>[4x]SRTDRLEVCREYQR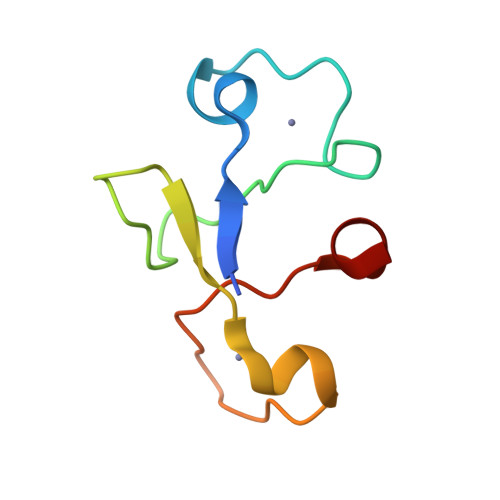GNCNRGENDCRFAHPADSTMIDTNDNTVTVCMDYIKGRCSREKCKYFHPPAHLQAK>HSVKLRPLEREDLRYVHQLDNNASVMRYWFEEPYEAFVELSDLYDKHIHDQSERRFVVECDGEKAGLVELVEINHVHRRAEFQIIISPEYQGKGLATRAAKLAMDYGFTVLNLYKLYLIVDKENEKAIHIYRKLGFSVEGELMHEFFI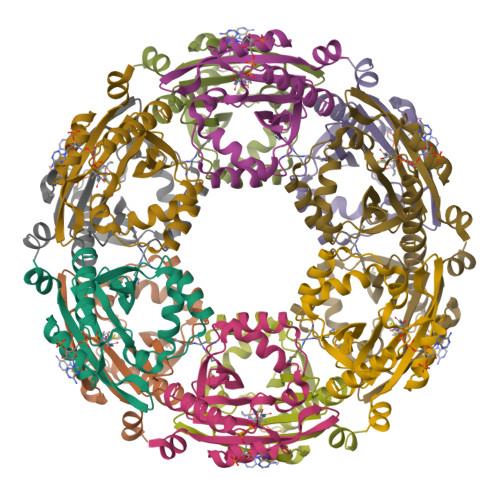NGQYRNAIRMCIFQHQYLAEHK[4x]2,4-bis(oxidanyl)-6-pentyl-benzoic acid | C12 H16 O4 | 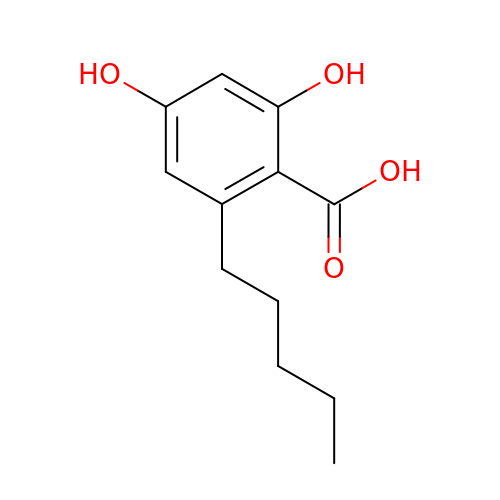SXFKFRRXJUJGSS-UHFFFAOYSA-N>[6x]GAMGSTVGLTALKVSGETLSEPMRPGVIRFGLTPVFLSNDLEVLDELQAYLTQAVGQEVQLITQRTYQEVTALLVSGNLEAAWICGYPFMKFRDELDLVATPLWRGKPVYQSYLIVGRDRDIAGFEDCQGDIHAFSDPDSNSGYLVTKTYLAERGVSEEGFFRKSFFTYGHRNVIRAVASGLADSGSVDGYVWEVMKTTEPELVAKTRVLVKSGWHGFPPVAAAAGQRKSQAVARIRSALLDMNQEVLGRSVLTRLQLDGFVETTAESYDSIAANMERVRRLG

The regulatory cluster consists of three genes, aioX, aioS and aioR, which encode a periplasmic-binding protein (PBP), a sensor histidine kinase and a response regulator, respectively. Arsenite-bound AioX is thought to act as a ligand for AioS, the sensor histidine kinase that upon auto-phosphorylation, phosphorylates AioR, the response regulator, which binds to a conserved sequence upstream of a RpoN promoter. AioX exhibits a typical bilobed structure of the PBP type II class. In this class of proteins, the ligand-binding pocket is located in the space between the two domains.

The crystal structure of the phosphate-bound AioX was used to solve the structures of the apo and arsenite-bound forms of the protein by molecular replacement. Figure 5 shows the AioX ligand-binding site with arsenite forming a link to the sulphur atom of Cys106, confirming the role of this residue in arsenite binding. While the majority of both structures overlay very well, there is a significant difference in the rotamer conformation of Tyr88. The change in the side chain conformation is further associated with the backbone shift for residues 83–88 and a significant conformational change in the loop region comprising residues 53–61, demarked by the black circle in Fig. 5A. Interestingly, while the structures of apo-AioX and the phosphate-bound AioX contained a monomer in the asymmetric unit, the arsenite-bound molecule crystallised with six molecules in the asymmetric unit of the unit cell. Although the six molecules were arranged as the three repeats of a loosely associated dimer none of the interfaces is sufficiently large to be indicative of a biologically significant assembly. The arsenite-bound crystal structure of AioX showed significant conformational changes compared with the apo and phosphate-bound structures, specifically in the loop of residues 53–61 and the shape, as well as electrostatic potential, of the protein surface. It is possible that these modifications allow its interaction with the sensor histidine kinase, AioS, leading to its activation. AioX and ArxX bound arsenite with a Kd of 177 and 311 nM, respectively and no interaction was detected with any of the other substrates tested (data not shown).>[2x]CUGGGCGG;>[2x]CCGCCUGG

We have obtained crystals of a racemic compound consisting of l- and d-RNA duplexes in which the enantiomers pack in the crystal lattice in an asymmetric manner and show differences in their structures, crystal contacts and interactions with the solvent. The crystals of d- and l-RNA duplexes (CUGGGCGG)-(CCGCCUGG) belong to space group P1 with the unit cell parameters a = 21.1 Å, b = 26.7 Å, c = 39.1 Å, α = 105.9°, β = 97.0°, and γ = 91.6°. The unit cell contains one d-RNA duplex and one l-RNA duplex stacking head-to-tail, arranged in the crystal lattice into parallel semi-infinite columns. The d-duplexes have the helical parameters characteristic of A-RNA, while the l-duplexes take values appropriately inverted for the other enantiomer.

The absolute configuration of the structure was determined for each analyzed crystal using the anomalous dispersion of X-rays from the Zn2+ ions. Of the nine crystals that gave diffraction data containing statistically significant anomalous signals, seven crystals had the K:L RNA duplex in the d-configuration, and the M:N duplex was in the l-configuration. The remaining two crystals had the inverted configuration l-(K:L)/d-(M:N). Of the eight crystals that gave no statistically significant anomalous signal but gave anomalous peaks at the Zn2+ ions, four crystals were d-(K:L)/l-(M:N), and four were l-(K:L)/d-(M:N). The ratio of the d-(K:L)/l-(M:N) to l-(K:L)/d-(M:N) crystal structures, of 7 to 2 for the best data sets and 11 to 6 overall, does not indicate a clear bias. The intermolecular crystal contacts of the two enantiomers are also different. When the two duplexes (K:L and M:N) are compared, chain K is more exposed to the solvent than its corresponding enantiomer, chain M, which makes more extensive contacts with neighboring RNA molecules. The percentage ratio of the solvent-exposed surface area to the intermolecular crystal contact area is 72/28 for chain K and 57/43 for chain M. The situation is reversed for the other strands of the two duplexes: the ratios of the solvent-exposed intermolecular contact areas are 55/45 for chain L and 71/29 for chain N. Asymmetry between the RNA enantiomers is also observed in their interactions with the Zn2+ ions. In the presented structure, one enantiomer interacts with three zinc cations, while the other interacts with four zinc cations.>[2x]SMRKSREYEHVRRDLDPNEVWEIVGELGDGAFGKVYKAKNKETGALAAAKVIETKSEEELEDYIVEIEILATCDHPYIVKLLGAYYHDGKLWIMIEFCPGGAVDAIMLELDRGLTEPQIQVVCRQMLEALNFLHSKRIIHRDLKAGNVLMTLEGDIRLADFGVSAKNLKTLQKRDSFIGTPYWMAPEVVMCETMKDTPYDYKAD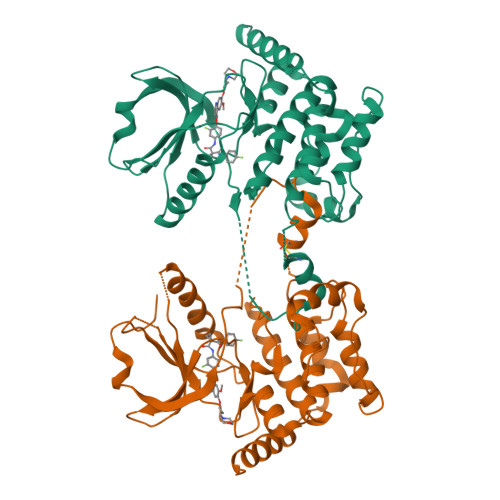IWSLGITLIEMAQIEPPHHELNPMRVLLKIAKSDPPTLLTPSKWSVEFRDFLAIALDKNPETRPSAAQLLEHPFVSSITSNKALRELVAEAKAEVMEE>[3x]MANAPHGGVLKDLLARDAPRQAELAAEAESLPAVTLTERQLCDLELIMNGGFSPLEGFMNQADYDRVCEDNRLADGNVFSMPITLDASQEVIDEKKLQAASRITLRDFRDDRNLAILTIDDIYRPDKTKEAKLVF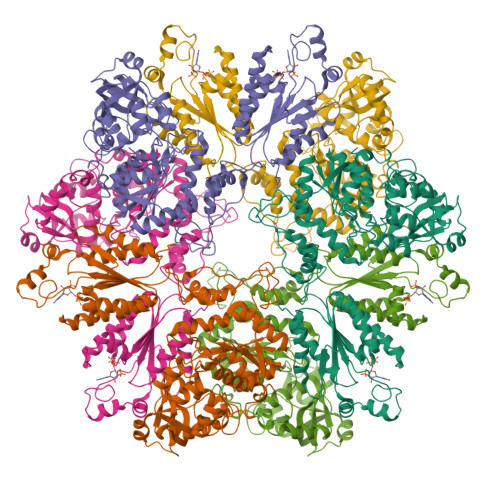GGDPEHPAIVYLNNTVKEFYIGGKIEAVNKLNHYDYVALRYTPAELRVHFDKLGWSRVVAFQTRNPMHRAHRELTVRAARSRQANVLIHPVVGLTKPGDIDHFTRVRAYQALLPRYPNGMAVLGLLGLAMRMGGPREAIWHAIIRKNHGATHFIVGRDHAGPGSNSKGEDFYGPYDAQHAVEKYKDELGIEVVEFQMVTYLPDTDEYRPVDQVPAGVKTLNISGTELRRRLRSGAHIPEWFSYPEVVKILRESNPPRATQGFTIFLTGYMNSGKDAIARALQVTLNQQGGRSVSLLLGDTVRHELSSELGFTREDRHTNIQRIAFVATELTRAGAAVIAAPIAPYEESRKFARDAVSQAGSFFLVHVATPLEHCEQSDKRGIYAAARRGEIKGFTGVDDPYETPEKADLVVDFSKQSVRSIVHEIILVLESQGFLERQ> MAKKTSSKGKLPPGPSPLPVLGNLLQMDRKGLLRSFLRLREKYGDVFTVYLGSRPVVVLCGTDAIREALVDQAEAFSGRGKIAVVDPIFQGYGVIFANGERWRALRRFSLATMRDFGMGKRSVEERIQEEARCLVEELRKSKGALLDNTLLFHSITSNIICSIVFGKRFDYKDPVFLRLLDLFFQSFSLISSFSSQVFELFPGFLKYFPGTHRQIYRNLQEINTFIGQSVEKHRATLDPSNPRDFIDVYLLRMEKDKSDPSSEFHHQNLILTVLSLFFAGTETTSTTLRYGFLLMLKYPHVTERVQKEIEQVIGSHRPPALDDRAKMPYTDAVIHEIQRLGDLIPFGVPHTVTKDTQFRGYVIPKNTEVFP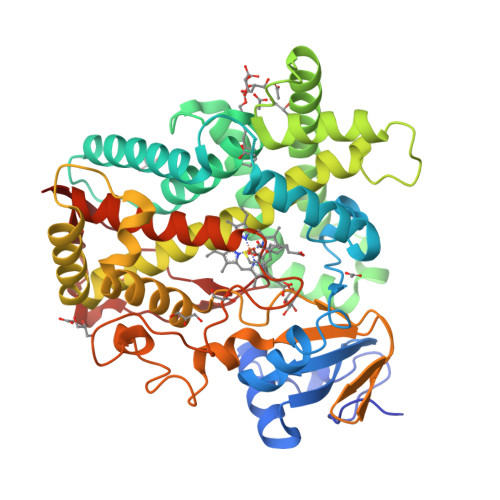VLSSALHDPRYFETPNTFNPGHFLDANGALKRNEGFMPHSLGKRICLGEGIARTELFLFFTTILQNFSIASPVPPEDIDLTPRESGVGNVPPSYQIRFLAR3-[N-[BENZYLOXYCARBONYL]-PHENYLALANINYL-AMINO]-5-PHENYL-PENTANE-1-SULFONIC 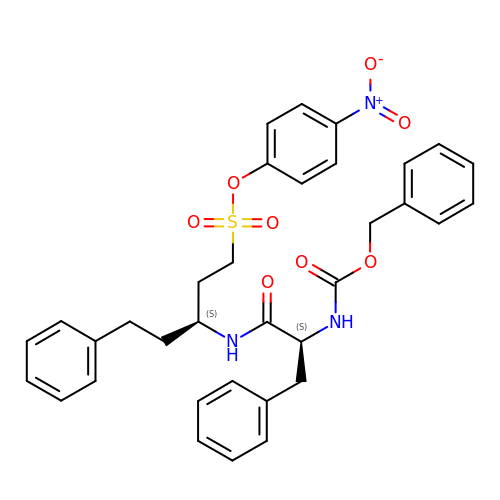ACID 4-NITRO-PHENYL ESTER | C34 H35 N3 O8 S | WABCRPSWXFHXDH-NYDCQLBNSA-N> MKCHRCGSDNVRKMVDSPVGDAWEVYV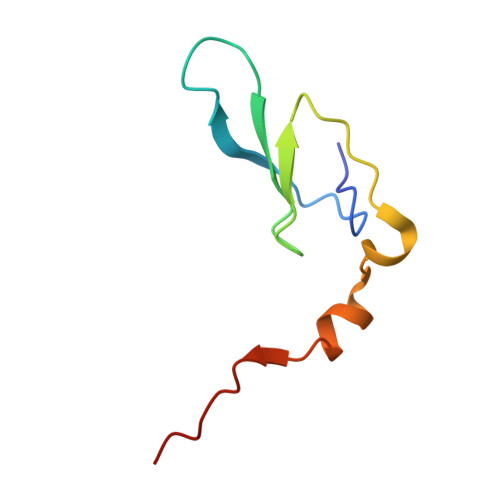CEKCCYSWRSTENPVVMEKFKLDDNKIANMGVIPPIPPLKK> MNQNLLVTKRDGSTERINLDKIHRVLDWAAEGLHNVSISQVELRSHIQFYDGIKTSDIHETIIKAAADLISRDAPDYQYLAARLAIFHLRKKAYGQFEPPALYDHVVKMVEMGKYDNHLLEDYTEEEFKQMDTFIDHDRDMTFSYAAVKQLEGKYLVQNRVTGEIYESAQFLYILVAACLFSNYPRETRLQYVKRFYDAVSTFKISLPTPIMSGVRTPTRQFSSCVLIECGDSLDSINATSSAIVKYVSQRAGIGINAGRIRALGSPIRGGEAFHTGCIPFYKHFQTAVKSCSQGGVRGGAATLFYPMWHLEVESL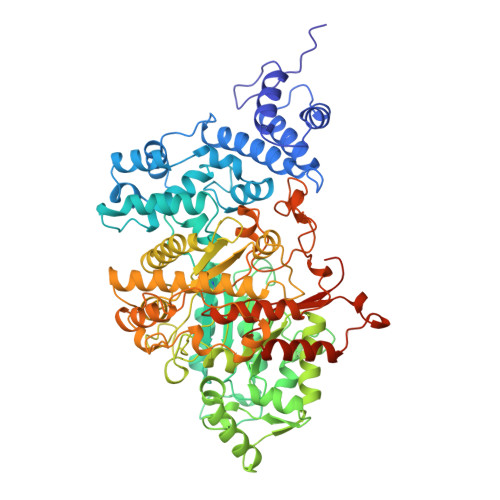LVLKNNRGVEGNRVRHMDYGVQINKLMYTRLLKGEDITLFSPSDVPGLYDAFFADQEEFERLYTKYEKDDSIRKQRVKAVELFSLMMQERASTGRIYIQNVDHCNTHSPFDPAIAPVRQSNLCLAIALPTKPLNDVNDENGEIALCTLSAFNLGAINNLDELEELAILAVRALDALLDYQDYPIPAAKRGAMGRRTLGIGVINFAYYLAKHGKRYSDGSANNLTHKTFEAIQYYLLKASNELAKEQGACPWFNETTYAKGILPIDTYKKDLDTIANEPLHYDWEALRESIKTHGLRNSTLSALMPSETSSQISNATNGIEPPRGYVSIKASKDGILRQVVPDYEHLHDAYELLWEMPGNDGYLQLVGIMQKFIDQSISANTNYDPSRFPSGKVPMQQLLKDLLTAYKFGVKTLYYQNTRDGAEDAQDDLVPSIQDDGCESGACKI2-(methylamino)-~{N}-[[4-[[2-(methylamino)ethanoylamino]methyl]phenyl]methyl]ethanamide | C14 H22 N4 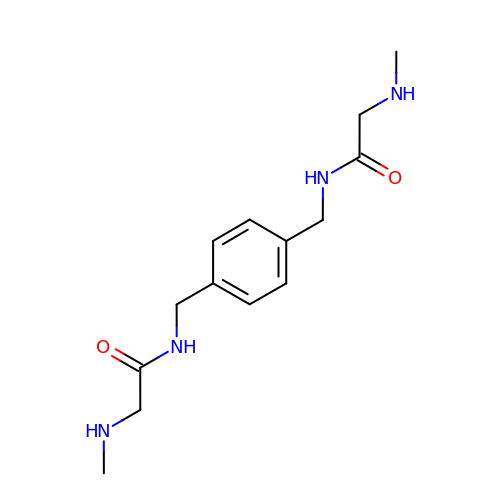O2 | RZNHDMVQBYDUNO-UHFFFAOYSA-N>GIDPFTTRPSSDLTAFREHFAKAKHIAIITGAGVSAESGVPTFRGPGGFWRKWQAQDLATPEAFSRDPSLVWEFYHYRREVMRSKMPNPAHLAIAECEARLGQQGRSVVIITQNIDELHHRAGSKHVYEIHGSLFKTRCMSCGEVKANHKSPICPALDGKGAPDPNTKEARIPVELLPRCERKSCNGLLRPHVVWFGETLDS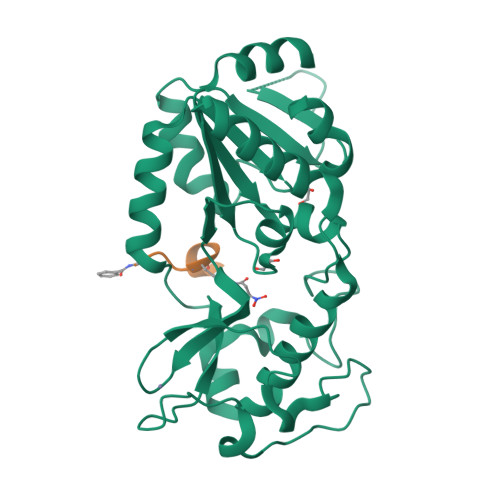DILTAVERELEKCDLCLVVGTSSIVYPAAMFAPQVASRGVPVAEFNMECTPATQRFKYHFEGPCGSTLPPALE[2x];> XGVLKEYGV> XVK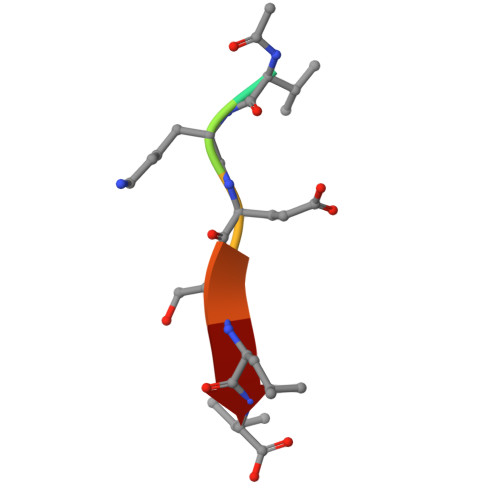ESLV>MDHVEETEILAATQRYYVERPIFSHPVLQERLHKKDKISESIGDKLKQAFTCTPKKIRNIIYMFLPITKWLPAYRFKEYVLGDIVSGISTGVLQLPQGLAFAMLAAVPPVFGLYSSFYPVIMYCFFGTSRHISIGPFAVISLMIGGVAVRLVPDDIVIPGGVNATNSTEARDALRVKVAMSVTLLTGIIQFCLGVCRFGFVAIYLTEPLVRGFTTAAAVHVFTSMLKYLFGVKTKRYSGIFSVVYSTVAVLQNVKNLNVCSLGVGLMVFGLLLGGKEFNERFKEKLPAPIPLEFFAVVMGTGISAGFSLHESYNVDVVGTLPLGLLPPANPDTSLFHLVYVDAIAIAIVGFSVTISMAKTLANKHGYQVDGNQELIALGLCNSTGSLFQTFAISCSLSRSLVQEGTGGKTQLAGCLASLMILLVILATGFLFESLPQAVLSAIVIVNLKGMFMQFSDLPFFWRTSKIELTIWLTTFVSSLFLGLDYGLITAVIIALMTVIYRTQSPSYIVLGQLPDTDVYIDIDAYEEVKEVPGIKIFQINAPIYYANSDLYSSALKRKTGVNPAFILGARRKAMKKYAKEVGNANMANATVVKVDAEVDAEDGTKPEEEEDEIKYPPIVTKSTLPEELQRFMPPGDNVHTIILDFTQVNFMDSVGVKTLAGIVKEYGDVGIYVYLAGCSAQVVSDLTQNQFFENPALLDLLFHSIHDAVLG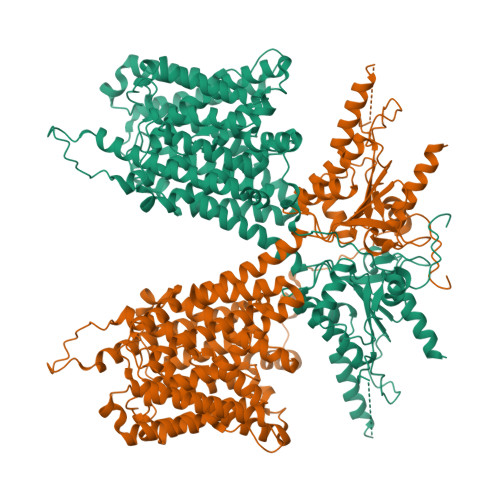SQVREALAEQEATAAPPQEDSEPNATPEA[2x]>MEKLHQCYWKSGEPQSDDIEASRMKRAAAKHLIERYYHQLTEGCGNEACTNEFCASCPTFLRMDNNAAAIKALELYKINAKLCDPHPSKKGASSAYLENSKGAPNNSCSEIKMNKKGARIDFKDVTYLTEEKVYEILELCREREDYSPLIRVIGRVFSSAEALVQSFRKVKQHTKEELKSLQAKDEDKDEDEKEKAACSAAAMEEDSEASSSRIGDSSQGDNNLQKLGPDDVSVDIDAIRRVYTRLLSNEKIETAFLNALVYLSPNVECDLTYHNVYSRDPNYLNLFIIVMENRNLHSPEYLEMALPLFCKAMSKLPLAAQGKLIRLWSKYNADQIRRMMETFQQLITYKVISNEFNSRNLVNDDDAIVAASKCLKMVYYANVVGGEVDTNHNEEDDEEPIPESSELTLQELLGEERRNKKGPRVDPLETELGVKTLDCRKPLIPFEEFINEPLNEVLEMDKDYTFFKVETENKFSFMTCPFILNAVTKNLGLYYDNRIRMYSERRITVLYSLVQGQQLNPYLRLKVRRDHIIDDALVRLEMIAMENPADLKKQLYVEFEGEQGVDEGGVSKEFFQLVVEEIFNPDIGMFTYDESTKLFWFNPSSFETEGQFTLIGIVLGLAIYNNCILDVHFPMVVYRKLMGKKGTFRDLGDSHPVLYQSLKDLLEYEGNVEDDMMITFQISQTDLFGNPMMYDLKENGDKIPITNENRKEFVNLYSDYILNKSVEKQFKAFRRGFHMVTNESPLKYLFRPEEIELLICGSRNLDFQALEETTEYDGGYTRDSVLIREFWEIVHSFTDEQKRLFLQFTTGTDRAPVGGLGKLKMIIAKNGPDTERLPTSHTAFNVLLLPEYSSKEKLKERLLKAITYAKGFGML[2x];>MHQKRTAMFQDPQERPRKLPQLCTELQTTIHDIILECVYCKQQLLRREVYDFAFRDLCIVYRDGNPYAVCDKCLKFYSKISEYRHYSYSLYGTTLEQQYNKPLSDLLIRCINCQKPLSPEEKQRHLDKKQRFHNIRGRWTGRCMSCSRSSRTRRETQL[2x]

Human protein E6AP/UBE3A, the founding member of the HECT-type ubiquitin ligase family, was originally identified as an associated partner of the viral oncoprotein E6 of human papillomaviruses (HPVs). The E6 oncoprotein from high-risk HPV types hijacks the ligase activity of the host E6AP to ubiquitinate the tumor suppressor p5313, leading to the aberrant p53 degradation. The HECT-type E3 ligases have a characteristic C-terminal HECT domain consisting of an N-lobe and a C-lobe that are responsible for E2 binding and ubiquitin acceptance, respectively. Here, by using cryogenic electronic microscopy, we reveal that the structures of full-length E6AP and E6AP/E6 complex are monomer and dimer of E6AP/E6 protomer, respectively.

After several rounds of 3D classification, we identified five distinct conformational states of the E6AP/E6 complex and resolved the structures of these five conformations at resolutions ranging from 2.6 to 4.4 Å. We therefore assigned the five conformations into one of two classes: attached (Att) or detached (Det). In all three Att conformations, the catalytic C-lobe of E6AP attaches to E6, whereas, in the two Det conformations, there are no interactions between the C-lobe and E6. We hereafter refer to the three Att conformations as Att1, Att2 and Att3 based on the distance between the tips of the two towers in a descending sequence: 74 Å in Att1, 71 Å in Att2, and 66 Å in Att3. Following the same nomenclature, the Det two conformations are referred to as Det1 (76 Å) and Det2 (61 Å). As the two towers underwent an outwards rotation, the Det2 conformation transformed into the Det1 conformation. Accompanying the E6AP/E6 complex conformational changes, there is substantial variation in the spatial relationship between the E6 from one protomer and the catalytic C-lobe of E6AP of the other protomer: far away (Det1), close (Det2), or in contact (Att). Among the five conformations, only the Det1 conformation showed the docked p53 core domain as being away from the inter-protomer C-lobe; the other four conformations showed clashes between the p53 core domain and the inter-protomer C-lobe. Therefore, we used the complex model of the E6AP/E6/p53 core domain, generated by docking p53 onto the E6AP/E6 structure of Det1, to investigate how E6AP/E6 protomeric dimerization contributes to p53 ubiquitination. The Det and Att conformations of the E6AP/E6 complex presented in this study should be structurally relevant to these accepting and donating processes, respectively. Unlike the N-lobe of E6AP, which is restricted by strong interactions with its N-terminal region, the C-lobe in the Det conformation is free to move around and accept ubiquitin from an E2; this is evident in the overlay structure of the HECT/E2–ubiquitin complex presented in Supplementary Fig. 14a.The first gene encodes the nucleoprotein (N protein) which associates with the viral genomic and antigenomic RNAs to form the helical nucleocapsid. The paramyxoviral nucleocapsid assembly entirely covers the viral genome, protecting it from detection and degradation by host factors and serving as the template for viral mRNA transcription and genome replication. Here, we determined the cryoEM structure of the recombinantly expressed, full-length, and tag-free HeV N protein in complex with E. coli host-derived RNA. Following cryoEM data collection, a multimeric HeV N protein double-ring assembly was resolved to 3.5 Å resolution, enabling the building and refinement of an atomic HeV N protein model.

The HeV Ncore structure follows the common bi-lobed paramyxoviral N protein fold and includes the Nt-arm (Met1-Thr32), NTD (Thr33-Glu260), CTD (Glu261-His370), and Ct-arm (His371-Ala394), as well as bound E. coli host-derived RNA. The cryoEM map of the HeV N protein assembly fully resolved the N protein core (Ncore), however no density was observed in the map corresponding to the intrinsically disordered C-terminal N protein tail (Ntail, Ala395-Val532). The N protein surface is overall hydrophilic, with three prominent hydrophobic patches that are covered by neighbouring N protomers in the assembly. The Nt-arm alpha helix (α1) contains a strongly negatively charged, solvent-exposed region facing the central cavity consisting of residues Asp3, Asp6, and Glu7. The HeV N assembly map showed clear density for single-stranded RNA in the RNA-binding cleft that separates the NTD and CTD, which was modelled as a poly-uridine; one hexa-uridine per N protomer. The RNA molecule is positioned in the conventional ‘three-base in, three-base out’ orientation, similar to other paramyxoviruses. In the case of HeV N, the 3’-most three-base stack is oriented in towards the RNA-binding cleft while the 5’-most three-base stack are oriented towards the solvent. The charged RNA-binding cleft consists of a cleft floor and two ridges that follow the orientation of the RNA chain. The cleft floor consists of the NTD-CTD-connecting loop Glu260-Ala265 continuing into α12 until Arg272 as well as the α14-containing stretch Ser317-Gly326. Within the RNA-binding cleft, a series of conserved basic (Lys178, Arg192, Arg193, Arg352) and polar (Thr181, Thr185, Gln199, Gln200, Tyr258, Gln319, Ser344, Tyr354) residues likely interact with the RNA chain through putative hydrogen bonds, salt bridges, and hydrophobic interactions.

> MSDIFDEAASFRSYQSKLGRDGRASAATATLTTKIRIFVPATNSPELRWELTLFALDVIRSPSAAESMKIGAAFTLISMYSERPGALIRSLLNDPDIEAVIIDVGSMLNGIPVMERRGDKAQEEMEGLMRILKTARESSKGKTPFVDSRAYGLRITDMSTLVSAVITIEAQIWILIAKAVTAPDTAEESETRRWAKYVQQKRVNPFFALTQQWLTEMRNLLSQSLSVRKFMVEILMEVKKGGSAKGRAVEIISDIGNYVEETGMAGFFATIRFGLETRYPALALNEFQSDLNTIKGLMLLYREIGPRAPYMVLLEESIQTKFAPGGYPLLWSFAMGVATTIDRSMGALNINRGYLEPMYFRLGQKSARHHAGGIDQNMANKLGLNSDQVAELAAAVQETSVGRQDNNMQAREAKFAAGGVLVGGGEQDIDEEEEPIEHSGRQSVTFKREMSMSSLADSVPSSSVSTSGGTRLTNSLLNLRSRLAAKAIKESTAQSSSERNPPNNRPQADSGRKDDQEPKPAQNDLDFVRADV> PPKRLTREAMRNYLKERGDQTVLILHAKVAQKSYGNEKRFFCPPPCVYLMGSGWKKKKEQMERDGCSEQESQPCAFIGIGNSDQEMQQLNLEGKNYCTAKTLYISDSDKRKHFMLSVKMFYGNSDDIGVFLSKRIKVISKPSKKKQSLKNADLCIASGTKVALFNRLRSQTVSTRYLHVEGGNFHASSQQWGAFYIHLLDDDESEGEEFTVRDGYIHYGQTVKLVCSVTGMALPRLIIRKVDKQTALLDADDPVSQLHKCAFYLKDTER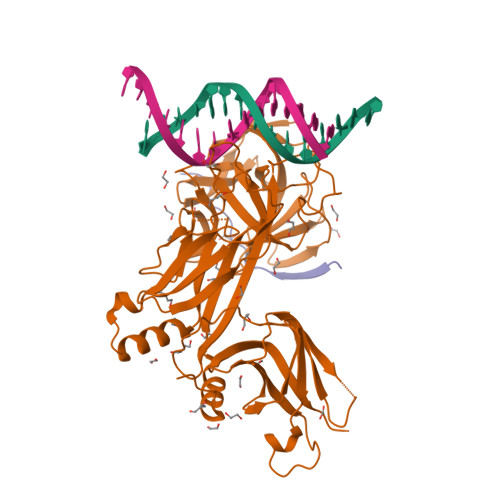MYLCLSQERIIQFQATPCPKEQNKEMINDGASWTIISTDKAEYTFYEGMGPVLAPVTPVPVVESLQLNGGGDVAMLELTGQNFTPNLRVWFGDVEAETMYRCGESMLCVVPDISAFREGWRWVRQPVQVPVTLVRNDGVIYSTSLTFTYTPEP;> DAAKLRALLWTPPPTP>MFTGSIVAIVTPMDEKGNVCRASLKKLIDYHVASGTSAIVSVGSTGESATLNHDEHADVVMMTLDLADGRIPVIAGTGANATAEAISLTQRFNDSGIVGCLTVTPYYNRPSQEGLYQHFKAIAEHTDLPQILYNVPSRTGCDLLPETVGRLAKVKNIIGIKEATGNLTRVNQIKELVSDDFVLLSGDDASALDFMQLGGHGVISVTANVAARDMAQMCKLAAEGHFAEARVINQRLMPLHNKLFVEPNPIPVKWACKELGLVATDTLRLPMTPITDSGRETVRAALKHAGLL[2x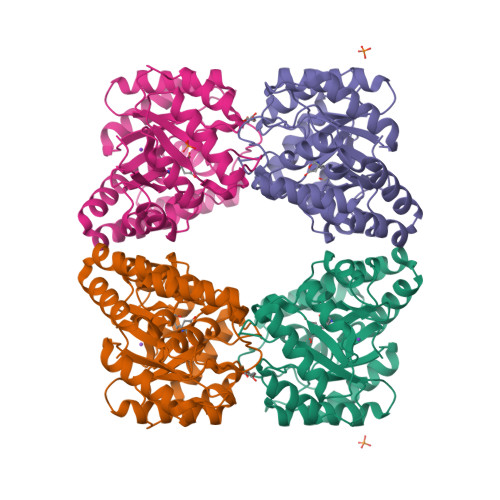]> MHHHHHHTRPDSKSMNYQLLKTFSRQPIQFGRFLARLLAGLVNTLKITRTSKSIELNLRIALPYLTPQQRIAITEKAVRNELTSYFEFLSIWGSSNSK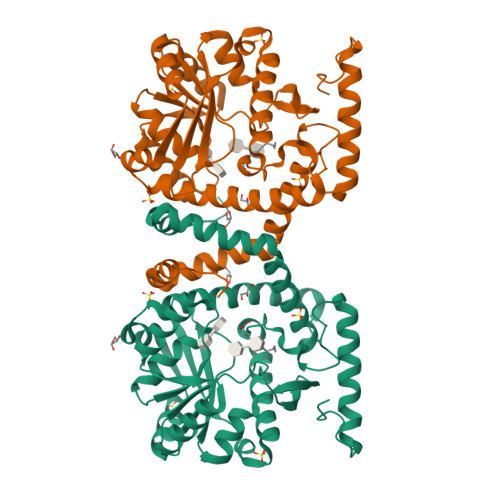NISRIHRIEGEHFFHEALAAKKGVVLIVPHFGTWAVMNAWCAQFTSMTILYKPVKNADADRFVREARSREQANLVPTDESGVRQIFKALKQGETTVILPDHTPNVGGDMVNYFGVPLASSNLSAKLIQKTKAKALFLYAIRNENDGFTMHIEPMDEKIYEGTADDGTYVIHQAIEQLIYQYPEHYHWSYKRFKANPALDNIYNIDPTEALKIVDRLKAEALKTSTQPEPIQTSVM EnvP(b)1 is an endogenous retroviral envelope gene found in human and other primate genomes. EnvP(b)1 has the characteristics of a classical gammaretroviral envelope protein. When ectopically expressed, human EnvP(b)1 can mediate fusion of cells in culture. EnvP(b)1 has all the hallmarks of a viral fusogen that has been repurposed to perform a host function.

We determined the crystal structure of the human EnvP(b)1 iRBD. Single anomalous dispersion (SAD) from a platinum derivative was used to obtain experimental phases and ultimately produce a model. The iRBD’s core is defined by a β sandwich that shares some similarity with a V-type Ig fold, although it lacks the first β sheet at the N terminus. Extensions between the β sheets form a series of loops and α-helical regions that decorate the core. There is weak sequence identity between these features and the gammaretrovirus variable regions A, B, and C (VRA, VRB, and VRC, respectively), which are believed to dictate Env-receptor interactions for gammaretroviruses. The iRBD shares little (∼20%) sequence identity with these examples, yet it shows extremely strong structural similarities. The EnvP(b)1 iRBD is more compact with shorter, less prominent loop structures extending from its core. All three VRs are shorter in EnvP(b)1: VRA and VRB are dramatically shorter, and the VRC, also shorter, adopts a different conformation as it is liberated from constraints by the absence of the paired Cys residues that form a disulfide in FrMLV and FeLV. As a consequence, the potential receptor-interacting interfaces of EnvP(b)1 are quite different from those for FrMLV and FeLV. The β sandwich core, a central helix that runs perpendicular to it, and an 8-amino-acid loop between the last two β sheets are all structurally conserved.

>[3x]ASHLIINVTRSDSPQTITFDACLVIPCGDLQSQRQLAAAEKYLCPSEADASTLFSFPFCHTWEYVVWTTQRQDWVPSQDFPLAVLKPYIHFTKGIAPPNCRYNQCNPVQISITIPTLQDSSPTLNRFYGMGADVRGKDPIGFFELHLSTSPSLISPRLSGAYPYDVPDYAGAGLEVLFQGPGGAHHHHHHHHGGAHHHHHH>[2x]GAMGSDSLVINLNRSNPKLKDLYIRPNIAQKRMQGSLEAHVNGFRFTSVRGDKVDILYNNIKHALFQPCDGEMIIVLHFHLKNA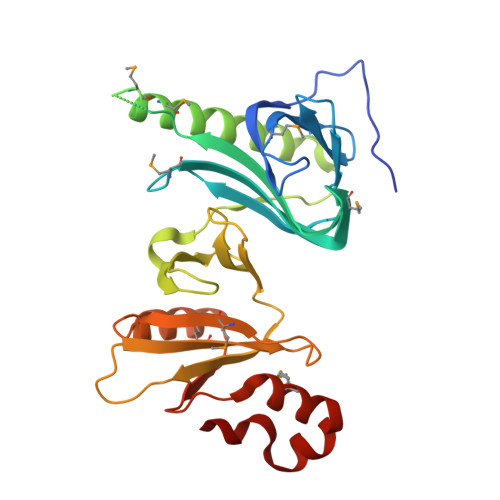IMFGKKRHTDVQFYTEVGEITTDLGKHQHMHDRDDLYAEQMEREMRHKLKTAFKNFIEKVEALTKEELEFEVPFRDLGFNGAPYRSTCLLQPTSSALVNATEWPPFVVTLDEVELIHFERVQFHLKNFDMVIVYKDYSKKVTMINAIPVASLDPIKEWLNSCDLKYTEGVQSLNWTKIMKTIVDDPEGFFEQGGWSFLE PMT-based O-mannosylation is an evolutionarily conserved and vital process, key for cell wall integrity and protein quality control in fungi. PMTs are divided into three subfamilies (PMT1, PMT2, and PMT4) and form functional dimers either within or across subfamilies (Akasaka-Manya et al., 2006; Girrbach and Strahl, 2003). In these structures each subunit has 11 transmembrane helices (TMHs) and two large hydrophilic loops oriented towards the ER lumen (LL): loop LL1 between TMH1 and 2 harboring a catalytic DE motif, and loop LL4 between TMH7 and 8, encompassing a so-called MIR domain, whose function remains unknown. MIR domains have a β-trefoil fold consisting of six β-hairpins arranged within a pseudo-threefold symmetry.

While MIR domains of the PMT1 family proved to be unstable when analyzed by nano differential scanning fluorimetry (nanoDSF) and failed to crystallize, PMT2 family MIR domains were more thermostable and readily formed crystals. X-ray structures were determined by molecular replacement using the MIR domain of the stromal-derived factor 2 (SDF2) from Arabidopsis thaliana previously solved in our laboratory (Radzimanowski et al., 2010; Schott et al., 2010). The high resolution of the Pmt2-MIR (1.6 Å) and Pmt3-MIR (1.9 Å) structures allowed for a detailed analysis of the respective structural properties and ligand interactions. An X-ray structure of the Pmt2-MIR has been reported in a parallel study but was not analyzed for carbohydrate-binding and functional implications. The MIR domains of the PMT2 family reveal the canonical β-trefoil fold (12 β-strands in total, PFAM trefoil clan CL0066, Figure 1C; Murzin et al., 1992), comprising a six-stranded β-barrel and a triangular β-hairpin cap including a hairpin triplet. Given the high sequence and structural similarity between Pmt2- and Pmt3-MIR domains (68% identity, rmsd of 0.7 Å for 194 Cα-atoms), we focused further analysis on the Pmt2-MIR domain. An almost identical arrangement is found for Pmt2-MIR site β in the MIRm1-MIRm2 interface. Both cavities are filled by ligands present in the crystallization solvent (glycerol in site α [also in Pmt3] and sulfate in site β). Taken together, we identified three putative ligand-binding sites in the Pmt2- and Pmt3-MIR domains. Two MIR-motifs form almost identical surface cavities and are conserved in all PMT-MIRs, while the third site is specific for MIRm3 of the PMT2 family and is highly solvent exposed. Our analysis of high-resolution X-ray structures of the Pmt2- and Pmt3-MIR domains revealed particular ligand-binding sites (α, β, δ) on each lateral side of the triangular cap region.

>[4x]MKHHHHHHPMGPRDVALGSSIISIKNQALGGALLHSHVQPFPEGSEQQQVTVYGYSDANNEWFFQRIRGVEPWTDAENKTIEFVKGGEMYRLMHRLTGKNLHTHEVPAPISKSEYEVSAYGDVDLGDYKDNWIIEIVEQVGEEDPTLLHPLSTSFRIKNSILGCYLAQSGKHLPEWGFRQGEVVCLKHASKRDKRTWWNIETHENERLPQGE>MELRHTPARDLDKFIEDHLLPNTCFRTQVKEAIDIVCRFLKERCFQGTADPVRVSKVVKGGSSGKGTTLRGRSDADLVVFLTKLTSFEDQLRRRGEFIQEIRRQLEACQREQKFKVTFEVQSPRRENPRALSFVLSSPQLQQEVEFDVLPAFDALGQWTPGYKPNPEIYVQLIKECKSRGKEGEFSTCFTELQRDFLRNRPTKLKSLIRLVKHWYQTCKKTHGNKLPPQYALELLTVYAWEQGSRKTDFSTAQGFQTVLELVLKHQKLCIFWEAYYDFTNPVVGRCMLQQLKKPRPV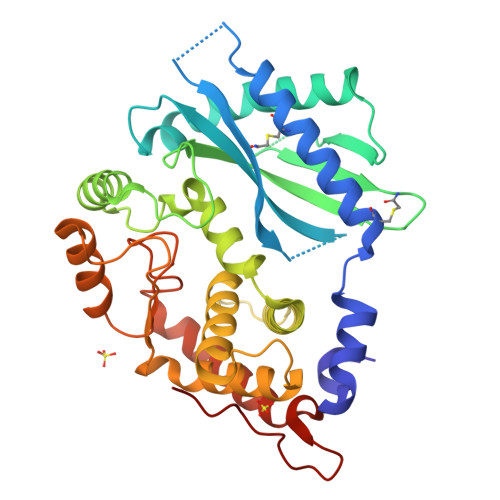ILDPADPTGNVGGGDTHSWQRLAQEARVWLGYPCCKNLDGSLVGAWTMLQKI[2x]>LSTSLSALPAAARDFVEEAVRLCRPREVLLCDGSEEEGKELLRGLQDDGVLHPLPKYDNCWLARTDPRDVARVESKTVLVTPEQSDAVPPPPPSGGPPQLGNWMSPNAFQAAVQERFPGCMAGRPLYVIPFSMGPPTSPLAKLGVQVTDSPYVVLSMRIMTRVGPAVLQRLDDDFVRCLHSVGRPLPLTEPLVSSWPCDPSRVLVAHIPSERRIVSFGSGYGGNSLLGKKCFALRIASRMAQQQGWLAEHMLILGVTSPSGEKRYMAAAFPSACGKTNLAMMTPSLPGWRIHCVGDDIAWMKFDDEGRLRAINPERGFFGVAPGTSSRTNPNAMATIARNTIFTNVGLRSDGGVYWDGLDEPTEPGVTYTSWLGKPWKHGDPEPCAHPNSRFCAPADQCPIMDPRWDDPEGVPIDAIIFGGRRPRGVPLVVEAFGWRHGVFMGSAMRSEATAAAEHKGGRLMHDPFAMRPFFGYNAGRYLEHWLSTGLRSNARLPRLFHVNWFLRDNEGRFVWPGFGHNARVLAWIFGRIQGRDT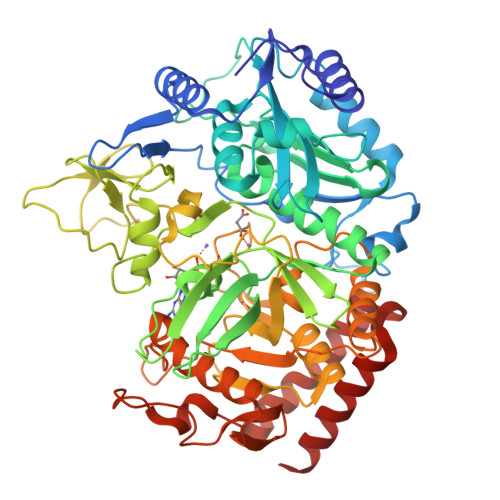ARPTPIGWVPKEGDLDLGGLPGVDYSQLFPMEKGFWEEECRQLREYYGENFGADLPRDVMAELEGLEERVRKM[4x]>[4x]AHLLTLNEATHEVQQVKLTRDQTSYGDEIDKFWLTQYVIHRESYDFYSV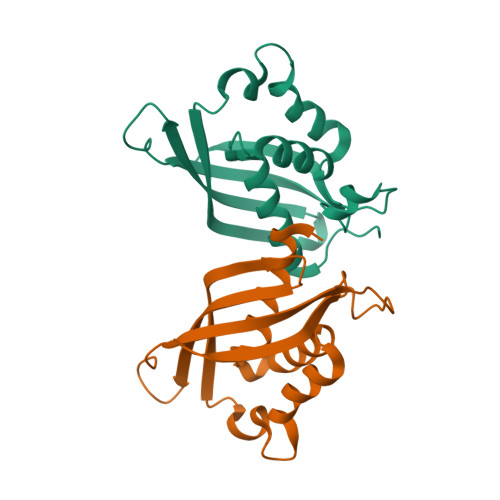QVDYTAVGLMSTPNVAESYQSKFKGRNGLDKVLGDSETTRVKINSVILDKPHGVATIRFTTVRRVRSNPVDDQPQRWIAIMGYEYKSLAMNAEQRYVNPLGFRVTSYRVNPEVN> AACCTACCTGGCAGGACGACTCTCTGCACTACTACGTCAGCA;> CACGAGCCTGATCGGACAAGA;> GAGCGACCTGTACGGACATCA;> TTTGCTGACGTAGTAGTGCAGAGAG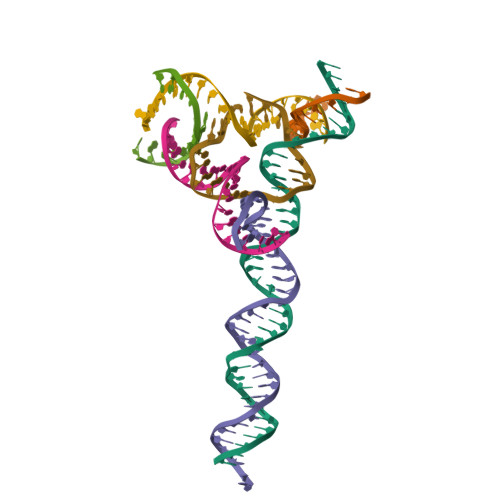TCGTGGCTCG;> TCTGATGTGGTAGG;> TGTCTTGTGGTCGC;> TACACCGATCACCTGCCACCG ethyl (6~{R})-3-oxidanylidenespiro[1,2,5,6-tetrahydropyrazolo[1,2-a]pyrazole-7,1'-cyclopentane]-6-carboxylate | 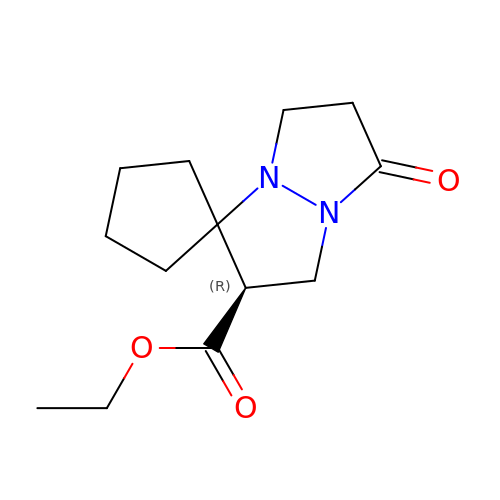C13 H20 N2 O3 | XBCGOHFXMUKNAT-JTQLQIEISA-N> MALYTPILILGAIAAVFAVVSVGI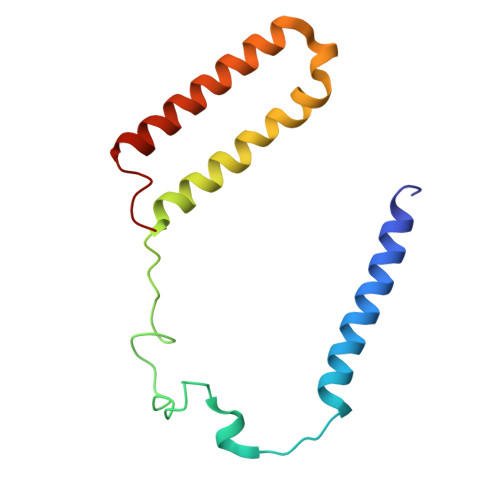ALVIGPRRFNRSKLEAYECGIDPLPPVAAGLTGQRIPIRYYLIAMLFIVFDIEIVFLYPWAVAFDSLGLFAVIEMLLFMLTVFVAYAYVWRRGGLNWD> ACYCRI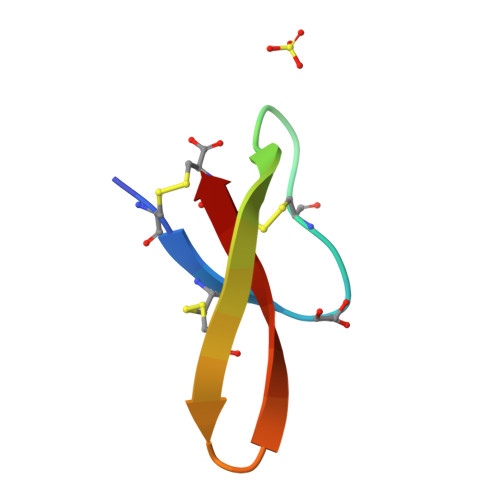PACIAGERRYGTCIYQGRLWAACC> RYKGGSPCISQPCLHNGSCQDSIWGYTCTCSPGYEGSNCELAKNECHPERTDGCQHFCLPGQESYTCSCAQGYRLGEDHKQCVPHDQCACGVLTSEKRAPDLQDLPWQVKLTNSEGKDFCGGVIIRENFVLTTAK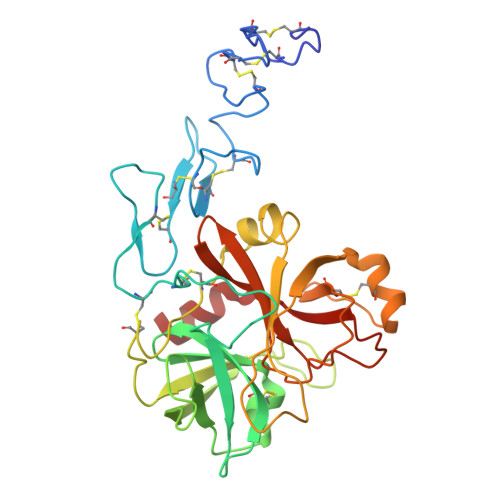CSLLHRNITVKTYFNRTSQDPLMIKITHVHVHMRYDADAGENDLSLLELEWPIQCPGAGLPVCTPEKDFAEHLLIPRTRGLLSGWARNGTDLGNSLTTRPVTLVEGEECGQVLNVTVTTRTYCERSSVAAMHWMDGSVVTREHRGSWFLTGVLGSQPVGGQAHMVLVTKVSRYSLWFKQIMN> MELIRIAMKKDLENDNSLMNKWATVAGLKNPNPLYDFLNHDGKTFNEFSSIVNIVKSQYPDREYELMKDYCLNLDVKTKAARSALEYADANMFFEIEDVLIDSMISCSNMKSKEYGKVYKIHRELSNSVITEFEAVKRLGKLNIKTPEMNSFSRLLLLYHYLSTGNFSPMAQLIKQIDLSEISENMYIRNTYQTRVHVLMSNIKLNENSLEECREYSKKALESTNILRFQVFSYLTIGNSLLFSNYELAQENFLK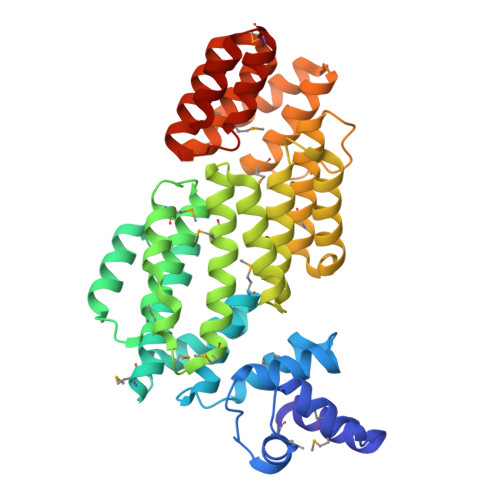GLSISVQNENYNMIFQQALCFLNNVWRKENKWINFESDSIMDLQEQAHCFINFNENSKAKEVLDKLDLLVHNDNELAMHYYLKGRLEQNKACFYSSIEYFKKSNDKFLIRLPLLELQKMGENQKLLELLLL> MGPSFNPVRFLELPIDIRKEVYFHLDGNFCGAHPYPIDILYKSNDVELPGKPSYKRSKRSKKLLRYMYPVFATYLNIFEYSPQLIEKWLEYAFWLRYDCLVLDCFKVNHLYDGTLIDALEWTYLDNELRLAYFNKASMLEVWYTFKEYK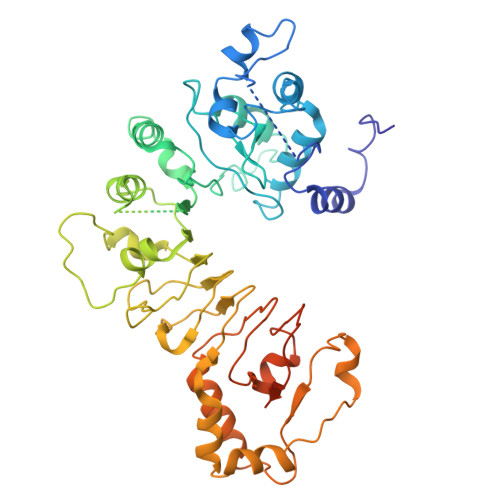KWVIDSVAFDELDLLNVSNIQFNIDNLTPQLVDKCLSILEQKDLFATIGEVQFGQDEEVGEEKDVDVSGANSDENSSPSSTIKNKKRSASKRSHSDNGNVGATHNQLTSISVIRTIRSMESMKSLRKITVRGEKLYELLINFHGFRDNPGKTISYIVKRRINEIRLSRMNQISRTGLADFTRWDNLQKLVLSRVAYIDLNSIVFPKNFKSLTMKRVSKIKWWNIEENILKELKVDKRTFKSLYIKEDDSKFTKFFNLRHTRIKELDKSEINQITYLRCQAIVWLSFRTLNHIKLQNVSEVFNNIIVPRALFDSKRVEIYRCEKISQVLVIGSRSGSENLYFQGSKRRWKKNFIAVSAANRFKKISSSGAL> DGFDAAAIGTQVANVIMGFVA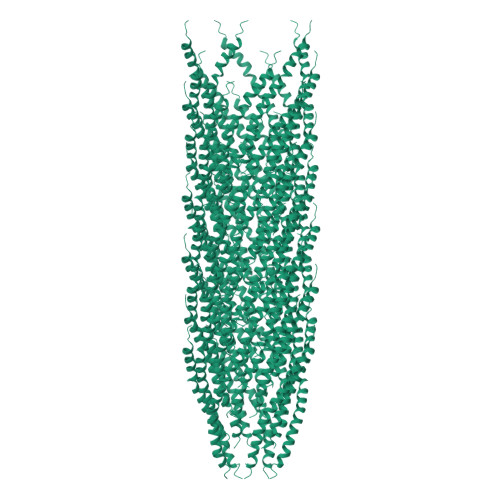MVSAVGMAAITVILAIQGFKMAWSMIKSVK> ETGNYMGNPWTEYMAKYDIEEVHGSGIRVDLGEDAEVAGTQYRLPSGKCPVFGKGIIIENSNTAFLTPVATGNQYLKDGGFAFPPTEPLMSPMTLDEMRHFYKDNKYVKNLDELTLCSRHAGNMIPDNDKNSNYKYPAVYDDKDKKCHILYIAAQENNGGGGGSGSDITQQAKDIGAGPVASCFTTRMSPPQQICLNSVVNTALSGGSGMFCFRPAKDISFQNYAYLSKNVVDNWEKVCPRKNLQNAKFGLWVDGNCEDIPHVNEFPAIDLFECNKLVFELSASDQPGGSGYKSHGKGYNWGNYNTETQKCEIFNVKPTCLINNAAYIATTALSHPIEVEGTKHHHHHH

The malaria merozoite protein apical membrane antigen 1 (AMA1) is critical for RBC invasion and is one of the most promising blood-stage vaccine candidates. AMA1 binds to RON2 through a surface exposed loop (RON2L) to anchor the parasite to the host cell membrane prior to internalization into a parasitophorous vacuole. Here, three single-component AMA1-RON2L immunogens were designed that retain the structure of the two-component AMA1-RON2L complex: one structure-based design (SBD1) and two insertion fusions. We determined the X-ray crystal structures of SBD1 and insertion fusion immunogens 2 and 3 to resolutions of 1.80 Å, 1.85 Å, and 2.10 Å, respectively.

Additionally, we created insertion fusion immunogens by inserting RON2L into an AMA1 loop proximal to the RON2L binding site. Insertion fusion immunogens 2 and 3 were constructed by replacing several amino acids in the DIf loop of AMA1 with RON2L and a flanking Gly/Ser linker. Immunogen 2 lacks amino acids 260-PRYCNKDESKRNS-272 of the DIf loop, including Cys263, consequently disrupting a disulfide bridge. The disordered DII loop was replaced with a Gly/Ser linker in both of these insertion fusion immunogens to prevent the potential displacement of the fused RON2L. In contrast, insertion fusion immunogens 2 and 3 retained the RON2L binding mode of the complex but displayed local distortions in loops near the vicinity of the insertion sites, resulting in Cα RMSDs of 0.381 over 232 C-alpha residues and 0.309 Å over 228 C-alpha residues, respectively. However, the IC50 values elicited by the insertion fusion immunogens 2 and 3 were 1.5-2-fold higher (i.e., less potent), and they were significantly different from that of the AMA1 DI-DII-RON2L complex (P < 0.005). Similar to AMA1 alone, the insertion fusion immunogens 2 and 3 produced potent strain-specific responses but were ineffective in inducing a broad immune response, possibly due to the insertion of RON2L in the DIf loop. This insertion results in a loss of strain-transcending functional activity, suggesting that either the local structural perturbations introduced by the insertion fusion disrupt strain-transcending epitopes or epitopes within the DIf loop contribute to protection breadth.>[6x]AAKKDYYAILGVPRNATQEE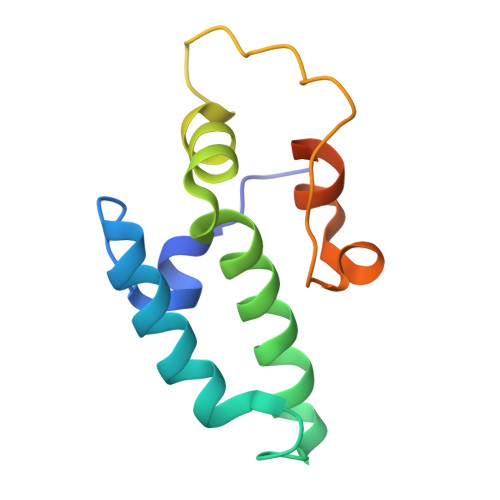IKRAYKRLARQYHPDVNKSPEAEEKFKEINEAYAVLSDPEKRRIYDTYGTTEAPPPPPPGGYDFSGFDVEDFSEFFQELFGPGLFGGFGRRSR>[6x]MPKQTLDGNTAAAHVAYAMSEVATIYPITPSSPMAEIADEWAAHGRKNIFGKTLQVAEMQSEAGAAGAVHGSLAAGALTTTFTASQGLLLMIPNMYKIAGELLPCVFHVAARALSTHALSIFGDHADVMAARQTGFAMLSSASVQEVMDLALVAHLATLKARVPFVHFFDGFRTSHEVQKIDVIEYEDMAKLVDWDAIRAFRQRALNPEHPHQRGTAQNPDIYFQSREAANPYYLATPGIVAQVMEQVAGLTGRHYHLFDYAGAPDAERVIVSMGSSCEVIEETVNYLVEKGEKVGLIKVRLFRPFSAEHFLKVLPASVKRIAVLDRTKEPGSLGEPLYEDVQTVLAEHGKNILVVGGRYGLGSKEFNPSMVKAVFDNLAATTPKNKFTVGITDDVTHTSLEIKEHIDTSPKGTFRCKFFGLGSDGTVGANKNSIKIIGDHTDMYAQGYFVYDSKKSGGVTISHLRFGKQPIQSAYLIDQADLIACHNPSYVGRYNLLEGIKPGGIFLLNSTWSAEEMDSRLPADMKRTIATKKLKFYNIDAVKIAQEIGLGSRINVIMQTAFFKIANVIPVDEAIKYIKDSIVKTYGKKGDKILNMNFAAVDRALEALEEIKYPASWADAVDEAAATVTEEPEFIQKVLRPINALKGDELPVSTFTPDGVFPVGTTKYEKRGIAVNIPQWQPENCIQCNQCSLVCPHAAIRPYLAKPADLAGAPETFVTKDAIGKEAAGLKFRIQVSPLDCTGCGNCADVCPAKVKAL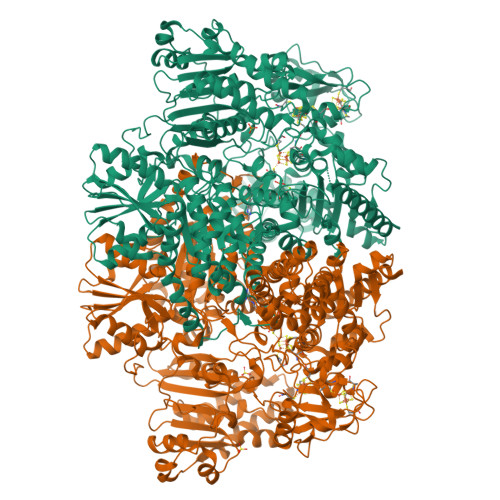TMVPLEEVTAVEEANYNFAEQLPEVKVNFNPATVKGSQFRQPLLEFSGACAGCGETPYVKLVTQLFGDRMIIANATGCSSIWGGSAPACPYTVNRQGHGPAWASSLFEDNAEFGYGMALAVAKRQDELATAISKALEAPVSAAFKAACEGWLAGKDDADRSREYGDRIKALLPGEISQASGEVKDLLLDIDRQKDYLTKKSIWIIGGDGWAYDIGYGGLDHVLASGANVNVLVLDTEVYSNTGGQSSKATQTGAVARFAAGGKFTKKKDLGLMAMSYGYVYVASVAMGASHSQLMKALIEAEKYDGPSLIIAYAPCINHGINMTYSQREAKKAVEAGYWPLYRYNPQLAQEGKNPFILDYKTPTASFRDFLMGEIRYTSLKKQFPEKAEQLFAKAEADAKARLEQYKKLAEG>MGSSHHHHHHGSFKDLNLTDAQKQQIREIMKGQRDQMKRPPLEERRAMHDIIASDTFDKAKAEAQIA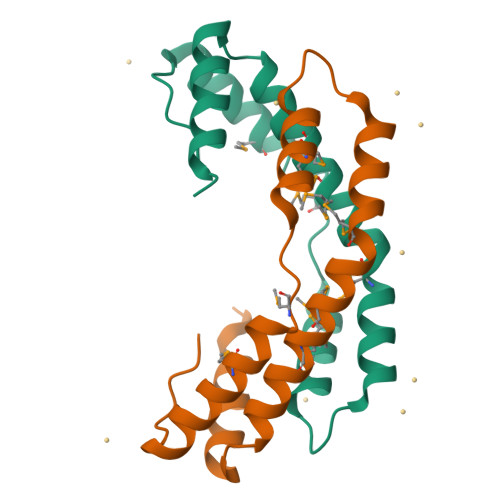KMEEQRKANMLAHMETQNKIYNILTPEQKKQFNANFEKRLT[2x]(1S,3R,6S)-4-oxo-6-{4-[(2-phenylquinolin-4-yl)methoxy]phenyl}-5-azaspiro[2.4]heptane-1-carboxylic acid | C29 H24 N2 O4 | 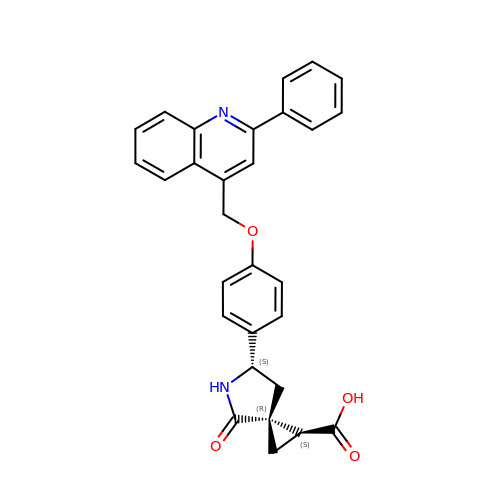BFZXMIUWGSTUAL-ZSOKXDGFSA-N> MMEYKIVENGLTYRIGNGASVPISNTGELIKGLRNYGPYEVPSLKYNQIALIHNNQFSSLINQLKSQISSKIDEVWHIHNINISEFIYDSPHFDSIKSQVDNAIDTGVDGIMLVLPEYNTPLYYKLKSYLINSIPSQFMRYDILSNRNLTFYVDNLLVQFVSKLGGKPWILNVDPEKGSDIIIGTGATRIDNVNLFCFAMVFKKDGTMLWNEISPIVTSSEYLTYLKSTIKKVVYGFKKSNPDWDVEKLTLHVSGKRPKMKDGETKILKETVEELKKQEMVSRDVKYAILHLNETHPFWVMGDPNNRFHPYEGTKVKLSSKRYLLTLLQPYLKRNGLEMVTPIKPLSVEIVSDNWTSEEYYHNVHEILDEIYYLSKMNWRGFRSRNLPVTVNYPKLVAGIIANVNRYGGYPINPEGNRSLQTNPWFL;> MGGSHHHHHHGMASENLYFQGGGGEIPLSSGNVNTPDVRSSGILYINIYPIVNYPETIKVSAIPYYEEFLPGKWKKRIGDLIYLYGYGIENEFDEIDNSNALFGKIFRKYLLDILSENIATPWQLKELGSTLRLVKEITENYEFSNIIKLQYELIINVHHWQNTNFGIIVDLKINILDRENNQRISYTKIKDKYGESVKKKIWVSVQAFHRHLTPEGKKYATAMRDKFNLLTGLLKEAFGSSEDEKTFSTPDGEIKIVFKPLEIVEVSNNDGI

Here we focus on the prokaryotic Argonaute AfAgo from Archaeoglobus fulgidus DSM4304. Although phylogenetically classified as a long-B pAgo, AfAgo contains only MID and catalytically inactive PIWI domains, akin to short pAgos. We show that AfAgo forms a heterodimeric complex with a protein encoded upstream in the same operon, which is a structural equivalent of the N-L1-L2 domains of long pAgos. This complex, structurally equivalent to a long PAZ-less pAgo, outperforms standalone AfAgo in guide RNA-mediated target DNA binding.

Next, we obtained cryo-EM structures of the fAfAgo complex with two variants of gRNA/tDNA heteroduplexes: g30/t51 (30 nt gRNA, 51 nt tDNA, final resolution 2.83 Å) and g17/t17 (17 nt gRNA, 17 nt gDNA, resolution 3.56 Å), and a 2.5 Å crystal structure of fAfAgo bound to a 15 nt 5′-phosphorylated ssDNA oligonucleotide. The nucleic acids resolved in the cryo-EM maps include a 25 bp protein-interacting fragment of gRNA/tDNA heteroduplex in the g30/t51 structure, and the full 17 bp gRNA/tDNA heteroduplex in the g17/t17 structure. fAfAgo proteins in these structures overlay with an RMSD value of ∼1.2 Å. We will base our further discussion of the fAfAgo structures on the higher resolution cryo-EM structure with the longer (g30/t51) gRNA/tDNA. The contact surface area between AfAgo and N-AfAgo proteins in this complex, as calculated by the PISA server, is 1380 Å2, and includes 15 H-bonds, indicative of stable association. Interestingly, the C terminus of AfAgo-N in the fAfAgo structure is adjacent to the N-terminus of Ago subunit, implying that both proteins could have evolved from a single polypeptide, and also accounting for the fully functional scfAfAgo fusion protein. The AfAgo-N subunit sterically masks the AfAgo surface that was previously implicated in AfAgo homodimerization, making AfAgo oligomerization across this surface unlikely. The overall structure of fAfAgo heterodimer aligns well with the structure of long-B Argonaute RsAgo. As predicted, AfAgo superimposes with MID and PIWI domains of RsAgo, whereas AfAgo-N superimposes with the N-terminal domain and the L1-L2 linker domains. Only the RsAgo PAZ domain has no structural counterpart in the fAfAgo complex. Similarly to RsAgo, fAfAgo binds the gRNA/tDNA heteroduplex in the positively charged cleft, which is formed by both AfAgo and AfAgo-N subunits, forming multiple van der Waals and H-bond interactions to the RNA/DNA backbone.>[2x]GMASIKGEVDE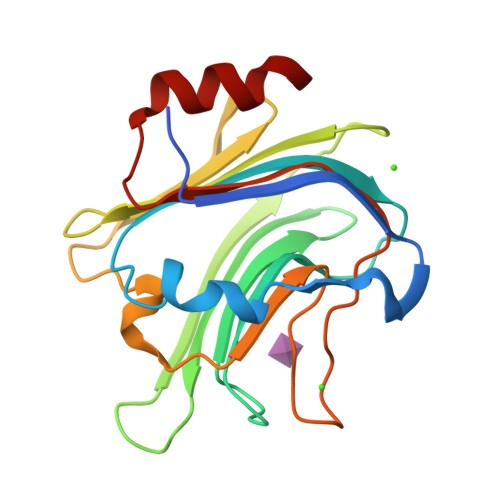IANYGNLKITKEEERVNITGDLEKFSSLEEGTIVTRFNMNDTSIQSLIGLSDGNKANNYFSLYVSGGKVGYELRRQEGNGDFNVHHSADVTFNRGINTLALKIEKGIGAKIFLNGSLVKTVSDPNIKFLNAINLNSGFIGKTDRANGYNEYLFRGNIDFMNIYDKPVSDNYLLRKTGETK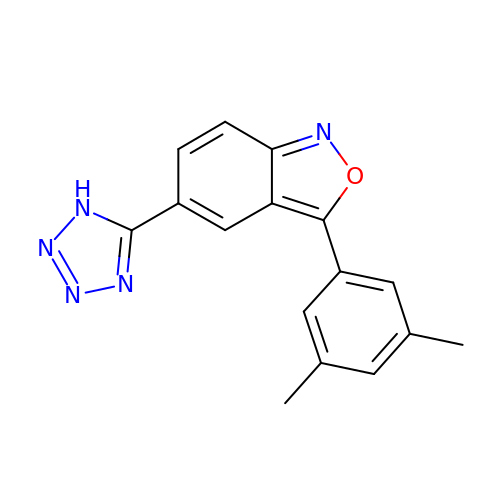(5P)-3-(3,5-dimethylphenyl)-5-(1H-tetrazol-5-yl)-2,1-benzoxazole | C16 H13 N5 O | PYDRHRMQZGFNTG-UHFFFAOYSA-N> ADGLYLQVGAFANPDAAELLKAKLSGVTAAPVFISSVVRNQQILHRVRLGPIGSADEVSRTQDSIRVANLGQPTLVRPD

However, it is known that the sporulation-related repeat (SPOR) domains (Pfam 05036), ubiquitous in prokaryotes, play a central role in directing proteins to the septum by recognition of the unique septal PG (rather than recognition by other division proteins), which is enriched in denuded glycans, the PG devoid of peptide stems. Of all SPOR-domain-containing proteins, RlpA is the most highly conserved across bacterial species, which underscores its important physiological role in bacteria. It is predicted to have two domains, a catalytic “double-ψ β-barrel” domain (DPBB; Pfam 03330) and a C-terminal SPOR domain. In the present report, we disclose the X-ray structure of the SPOR domain of rare lipoprotein A (RlpA) from P. aeruginosa (SPOR-RlpA).

The structure provided superb electron density for amino acids 265–342 of RlpA. The domain assembles into a concave four-stranded antiparallel β-sheet, complemented on one side by two α-helices. The β1 strand forms the central part of the fold with the adjacent β3 arranged in an antiparallel manner, and β4 and β2 contacting β1 and β3, respectively. As in other SPOR domains, the SPOR-RlpA domain is assembled by two repeats. The first repeat (residues 264–303) comprises β1, α1, and β2, while the second repeat (residues 304–342) comprises β3, α2, and β4. Numerous contacts are found between the two repeats. In addition to the hydrogen-bonding network between the β-strands, hydrophobic interactions play an essential role in linking the two repeats in a single compact structure. (i) There is no discernable conformational change in the backbone of the SPOR domain upon ligand binding (rmsd of 0.27 Å for Cα superimposition of SPOR domain alone and in complex with 1). Therefore, our results do not support the existence of “open” and “closed” conformations as a general mechanism in SPOR domain recognition, as previously proposed. Changes only concern side chains of residues R302 and R309, which offer two distinct conformations with direct involvement in ligand recognition and F274 that slightly changes its orientation upon ligand binding.(2S,3S,4R,5R,6R)-5-acetamido-6-[[[(2R,3S,4R,5R)-5-(2,4-dioxopyrimidin-1-yl)-3,4-dihydroxy-oxolan-2-yl]methoxy-hydroxy-phosphoryl]oxy-hydroxy-phosphoryl]oxy-3,4-dihydroxy-oxane-2-carboxylic 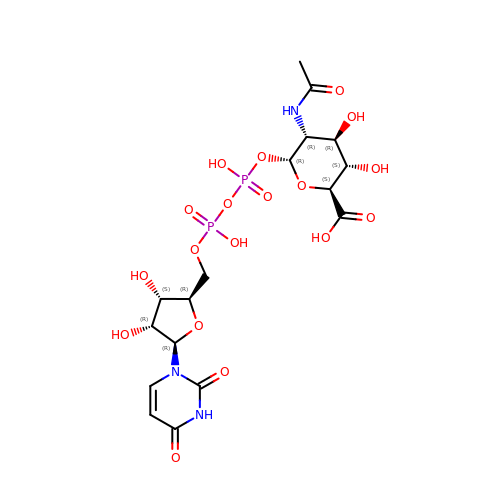acid | C17 H25 N3 O18 P2 | DZOGQXKQLXAPND-HHKCBAECSA-N>MFLTAEDSFELGKVAYTEADYYHTELWMEQALRQLDEGEISTIDKVSVLDYLSYAVYQQGDLDKALLLTKKLLELDPEHQRANG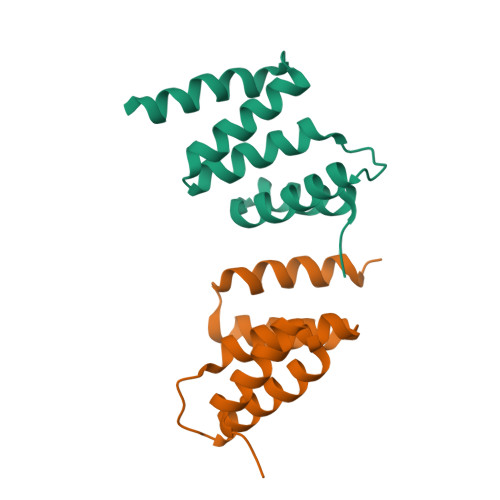NLKYFEYIMAKEKDVNKSHHHHHH[2x]> YFGKLESKLSVIRNLNDQVLFIDQGNRPLFEDMTDSDSRDNAPRTIFIISMYKDSQPRGMAVTISVKSEKISTLSSENKIISFKEMNPPDNIKDTKSDIIFFQRSVPGHDNKMQFESSSYEGYFLCSEKERDLFKLILKKEDELGDRSC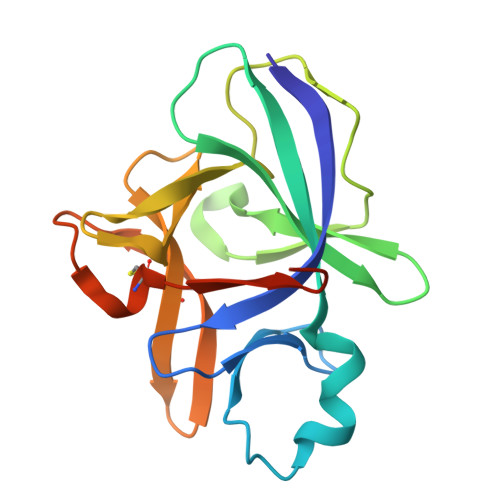MFTVQNEDGGGENLYFQ>[8x]GPHMDTKIIYHMDEEETPDLVKLPVAPERVT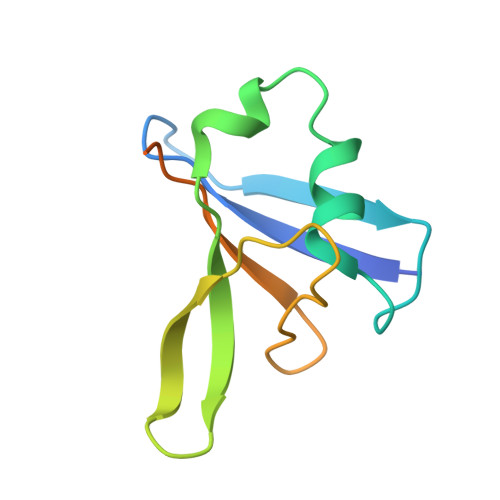LADFKNVLSNRPVHAYKFFFKSMDQDFGVVKEEIFDDNAKLPCFNGRVVSWLVLAEGAHSDAGSQGTDSHTDLPP We report here the crystal structure of a native and complexed lectin isolated from Canavalia gladiata seeds, describing a new binding pocket in ConA-like lectins, which may be related to pathogen resistance, a site where a non-protein amino acid, such as α-amino butyric acid, can bind. The most recent accepted definition establishes lectins as proteins with at least one non-catalytic domain able to recognize and bind reversibly to specific mono and oligosaccharides. The oligomeric structures of CGL and CGL-αMM involve two 'canonical' dimers, and these dimers are associated by salt bridges between β-strands. In both CGL crystal structures, the amino acids involved in metal binding are conserved.

The model was examined by Xfit, and one region around Asp 139 showed a well-defined electron density (fo-fc contoured at 5σ), not elucidated for the model, the atomic coordinates for this structure were deposited without the elucidation of this density with PDB access 1 WUV. After an analysis of the amino acid and secondary metabolite content in leguminous seeds, α-aminobutyric acid (Abu), a non-protein amino acid, was chosen according to electron density. Previous ConA structures showed some poor density regions at N-terminal residues and in surface loops at residues 118–122, 149–151, 160–163. The CGL structure presents well-defined electron density in these loops and is the first ConA-like structure that shows a stable loop in 118–122 region. The presence of Abu in the CGL structure was confirmed by mass spectrometry.

>ADTIVAVELDTYPNTDIGDPNYPHIGIDIKSVRSKKTAKWNMQNGKVGTAHIIYNSVGKRLSAVVSYPNGDSATVSYDVDLDNVLPEWVRVGLSASTGLYKETNTILSWSFTSKLKSNSTHETNALHFMFNQFSKDQKDLILQGDATTGTDGNLELTRVSSNGSPQGSSVGRALFYAPVHIWESSAVVASFDATFTFLIKSPDSHPADGIAFFISNIDSSIPSGSTGRLLGLFPDAN[4x]> SLSKDDTAQLKITNIEGGPTVTLYKIGEGVYNTNGDSFINFKYAEGVSLTETGPTSQEITTIANGINTGKIKPFSTENVSISNGTATYNARGASVYIALLTGATDGRTYNPILLAASYNGEGNLVTKNIDSKSNYLYGQTSVAKSSLPSITKKVTGTIDDVNKKTTSLGSVLSYSLTFELPSYTKEAVNKTVYVSDNMSEGLTFNFNSLTVEWKGKMANITEDGSVMVENTKIGIAKEVNNGFNLSFIYDSLESISPNISYKAVVNNKAIVGGEGNPNKAEFFYSNNPTKGNTYDNLDKKPDKGNGITSKEDSKIVYTYQIAFRKVDSVSKTPLIGAIFGVYDTSNKLIDIVTTNKNGYAISTQVSS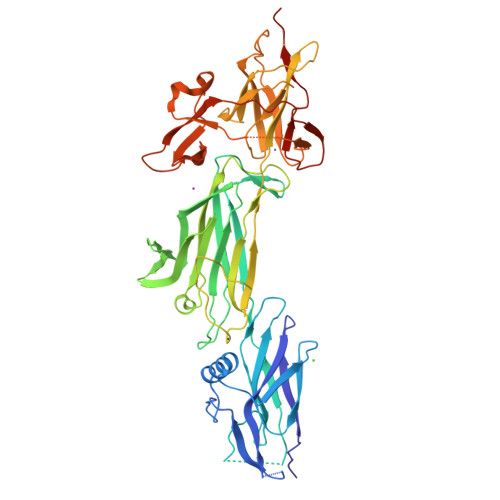GKYKIKELKAPKGYSLNTETYEITANWVTATVKTSANSKSTTYTSDKNKATDNSEQVGWLKNGIFYSIDSRPTGNDVKEAYIESTKALTDGTTFSKSNEGSGTVLLETDIPNTKLGELPSTG>[2x]MILKRAYDVTPQKISTDKIRGVHKRVLIGLKDAPNFVIRLFTVEPGG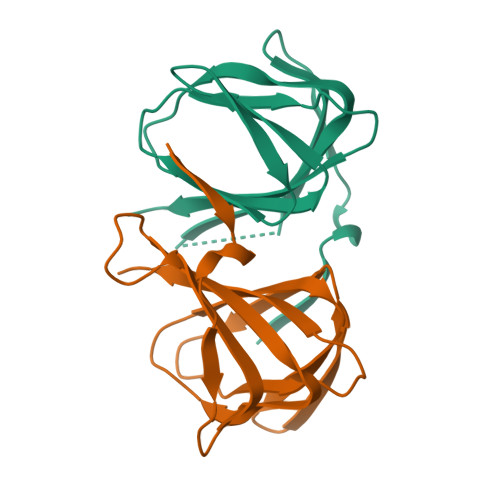LIDRHSHPWEHEFFVLKGKLTVLKEQGEETVEEGFYIFVEPNEIHGFRNDTDSEVEFLQLIPKEGGE> DPHSETAL;> LLIEPARIEEEELTLTILRQTGGLGISIAGGKG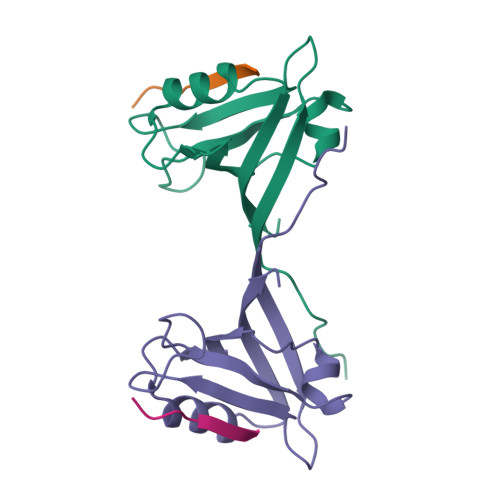STPYKGDDEGIFISRVSEEGPAARAGVRVGDKLLEVNGVALQGAEHHEAVEALRGAGTAVQMRVWRERM>FEGDLKWHHHNITYWIQNYSEDLPRAVIDDAFARAFALWSAVTPLTFTRVYSRDADIVIQFGVAEHGDGYPFDGKDGLLAHAFPPGPGIQGDAHFDDDELWSLGKGVGYSLFLVAAHEFGHALGLDHSSVPEALMYPMYRFTEGPP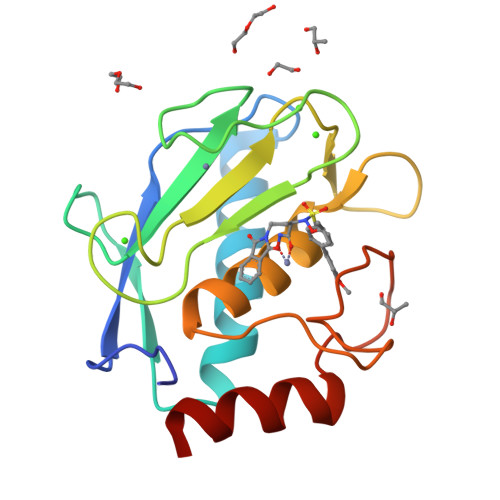LHKDDVNGIRHLYG[2x]>[7x]MKTDDKDREGGDSHGAIGAKLMEYALK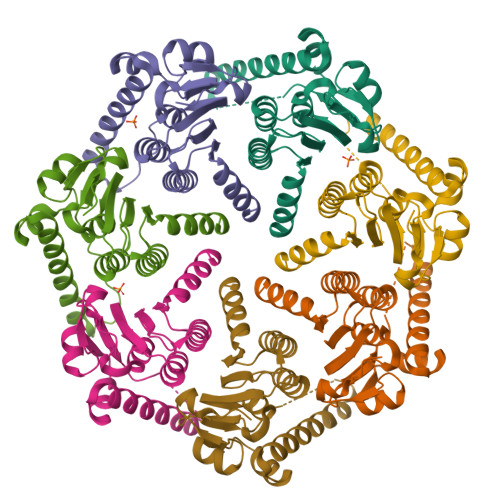VRKVFVTGGVDEKMAKDVVQQLHILASISDDPIYMFVNSPGGHVESGDMIFDAIRFITPKVIMIGSGSVASAGALIYAAADKENRYSLPNTRFLLHQPSGGIQGPASNIEIYRREIVRMKERLDRIFAEATGQTPEKISADTERDFWLNAEEAVQYGLVNKIIVSEREITLPGQSGWSHPQFEK5-[(1Z)-2-(2-methoxyphenyl)prop-1-en-1-yl]furo[2,3-d]pyrimidine-2,4-diamine | C16 H16 N4 O2 | 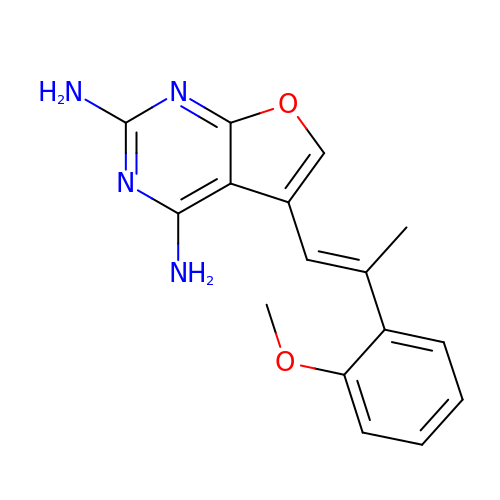JXICVPBZQSPDOK-CLFYSBASSA-N>[2x]MPAVTQPRGESKYDAIPGPLGPQSASLEGKVALVTGAGRGIGREMAMELGRRGCKVIVNYANSTESAEEVVAAIKKNGSDAACVKANVG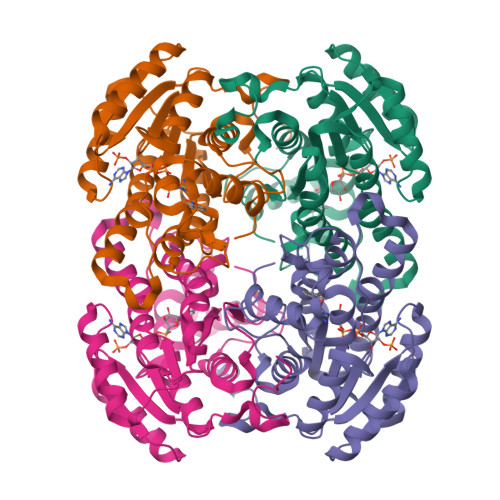VVEDIVRMFEEAVKIFGKLDIVCSNSGVVSFGHVKDVTPEEFDRVFTINTRGQFFVAREAYKHLEIGGRLILMGSITGQAKAVPKHAVYSGSKGAIETFARCMAIDMADKKITVNVVAPGGIKTDMYHAVCREYIPNGENLSNEEVDEYAAVQWSPLRRVGLPIDIARVVCFLASNDGGWVTGKVIGIDGGACM> AKFELPELPYAYDALEPTIDKETMNIHHTKHHNTYVTKLNGALEGHEDLKNKSLNDLISNLDAVPENIRTAVRNNGGGHANHSLFWKLMSPNGGGKPTGEVADKINDKYGSFEKFQEEFAAAAAGRFGSGWAWLVVNNGEIEIMSTPIQDNPLMEGKKPILGLDVWEHA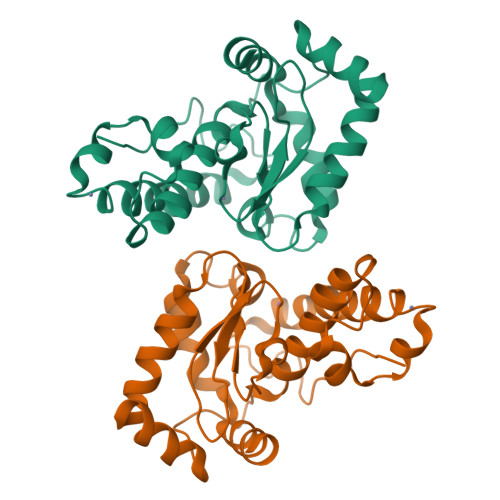YYLKYQNKRPDYISAFWNVVNWDEVAAQYSQAA> QCYHGNGQSYRGTFSTTVTGRTCQSWSSMTPHRHQRT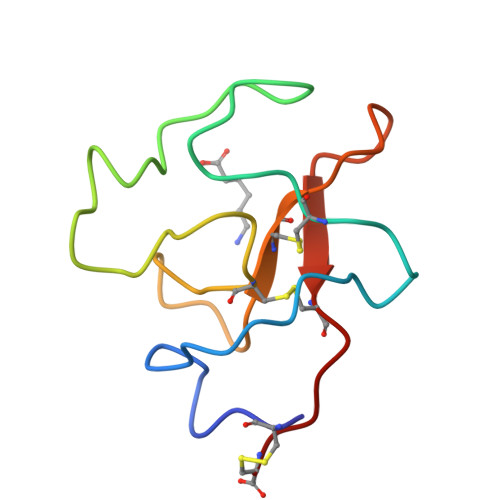PENYPNDGLTMNYCRNPDADTGPWCFTTDPSIRWEYCNLTRC> PISPIETVPVKLKPGMDGPKVKQWPLTEEKIKALVEICTEMEKEGKISKIGPENPYNTPVFAIKKKDSTKWRKLVDFRELNKRTQDFWEVQLGIPHPAGLKKKKSVTVLDVGDAYFSVPLDEDFRKYTAFTIPSINNETPGIRYQYNVLPQGWKGSPAIFQSSMTKILEPFKKQNPDIVIYQYIDDLYVGSDLEIGQHRTKIEELRQHLLRWGLTTPDKKHQKEPPFLWMGYELHPDKWTVQPIVLPEKDSWTVNDIQKLVGKLNWASQIYPGIKVRQLSKLLRGTKALTEVIPLTEEAELELAENREILKEPVHGVYYDPSKDLIAEIQKQG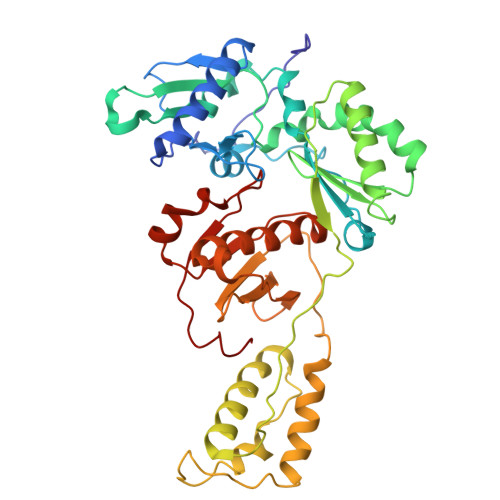QGQWTYQIYQEPFKNLKTGKYARMRGAHTNDVKQLTEAVQKITTESIVIWGKTPKFKLPIQKETWETWWTEYWQATWIPEWEFVNTPPLVKLWY>GSITENTSWNKEFSAEAVNGVFVLCKSSSKSCATNDLARASKEYLPASTFKIPNAIIGLETGVIKNEHQVFKWDGKPRAMKQWERDLTLRGAIQVSAVPVFQQIAREVGEVRMQKYLKKFSYGNQNISGGIDKFWLEGQLRISAVNQV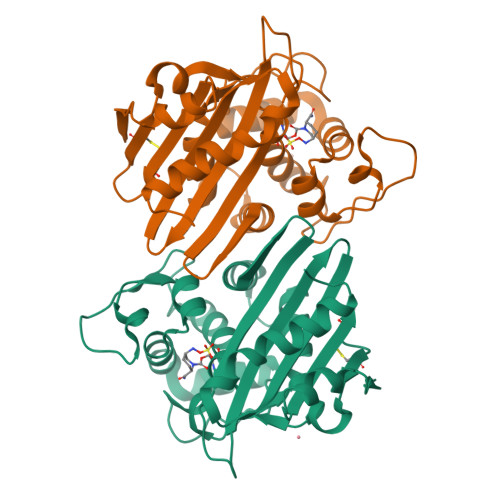EFLESLYLNKLSASKENQLIVKEALVTEAAPEYLVHSKTGFSGVGTESNPGVAWWVGWVEKETEVYFFAFNMDIDNESKLPLRKSIPTKIMESEGIIG[2x]>SSPGKPPRLVGGPMDASVEEEGVRRALDFAVGEYNKASNDMYHSRALQVVRARKQIGAGVNYFLDVELGRTTCTKTQPNLDN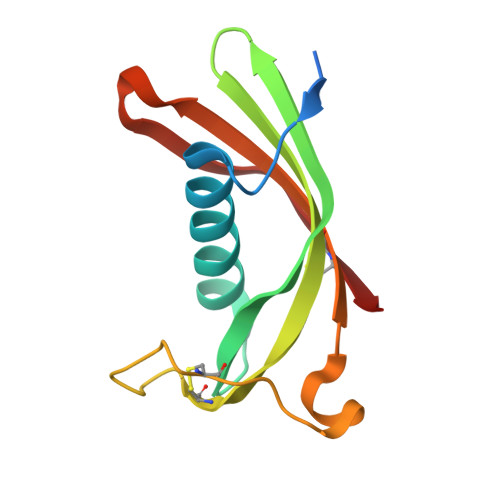CPFHDQPHLKRKAFCSFQIYAVPWQGTMTLSKSTCQDA[2x]>MGSITENTSWNKEFSAEAVNGVFVLCKSSSKSCATNDLARASKEYLPASTFKIPNAIIGLETGVIKNEHQVFKWDGKPRAMKQWERDLTLRGAIQVSATPVFQQIAREVGEVRMQKYLKKFSYGNQNISGGIDKFWLEGQLRISAVNQVEFLESLYLNKLSASKENQLIVKEALVTEAAPEYLVHSKTGFSGVGTESNPGVAWWVGWVEKETEVYFFAFNMDIDNESKL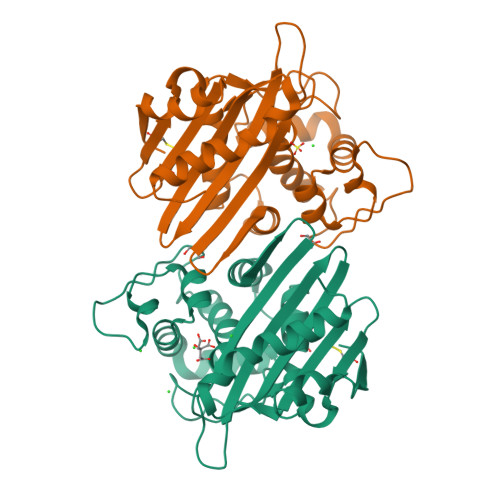PLRKSIPTKIMESEGIIGG[2x]>GPLGSTMEQKTVIPGMPTVIPPGLTREQERAYIVQLQIEDLTRKLRTGDLGIPPNPEDRSPSPEPIYNSEGKRLNTR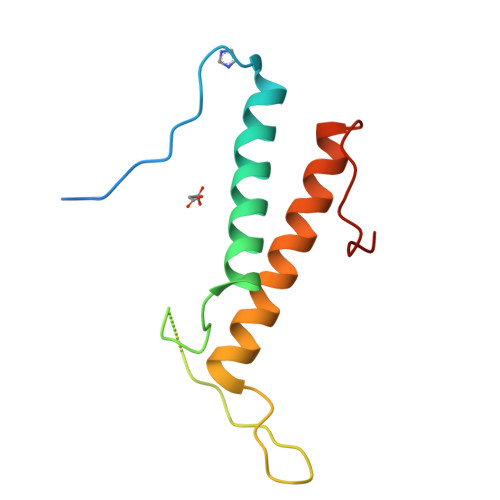EFRTRKKLEEERHNLITEMVALNPDFKPPADYKPP[4x]> QEVEFDIPPQALGSALQEFGRQADIQVLYRPEEVRNKRSSAIKGKLEPNQAITELLRGTGASVDFQGNAITISVAEAADSSVDLGATMITSNQLGTITEDSGSYTPGTIATATRLVLTPRETPQSITVVTRQNMDDFGLNNIDDVMRHTPGITVSAYDTDRNNYYARGFSINNFQYDGIPSTARNVGYSAGNTLSDMAIYDRVEVLKGATGLLTGAGSLGATINLIRKKPTHEFKGHVELGAGSWDNYRSELDVSGPLTESGNVRGRAVAAYQDKHSFMDHYERKTSVYYGILEFDLNPDTMLTVGADYQDNDPKGSGWSGSFPLFDSQGNRNDVSRSFNNGAKWSSWEQYTRTVFANLEHNFANGWVGKVQLDHKINGYHAPLGAIMGDWPAPDNSAKIVAQKYTGETKSNSLDIYLTGPFQFLGREHELVVGTSASFSHWEGKSYWNLRNYDNTTDDFINWDGDIGKPDWGTPSQYIDDKTRQLGSYMTARFNVTDDLNLFLGGRVVDYRVTGLNPTIRESGRFIPYVGAVYDLNDTYSVYASYTDIFMPQDSWYRDSSNKLLEPDEGQNYEIGIKGEYLDGRLNTSLAYFEIHEENRAEEDALYNSKPTNPAITYAYKGIKAKTKGYEAEISGELAPGWQVQAGYTHKIIRDDSGKKVSTWEPQDQLSLYTSYKFKGALDKLTVGGGARWQGKSW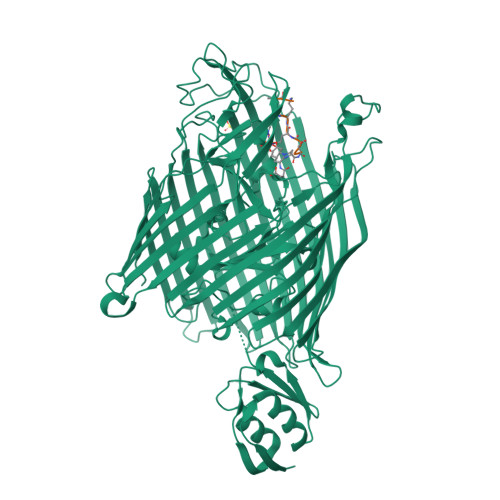QMVYNNPRSRWEKFSQEDYWLVDLMARYQITDKLSASVNVNNVFDKTYYTNIGFYTSASYGDPRNLMFSTRWDF;> SRSKKKTT> GSHMRIDPFKLAHWMNARKYTAAQTADLAGLPLDDLRRLLGDEANEPDPAAATALAEALSVEPSQLAADAHRNLTVVHKSAEEMHASRRPIQRDGIHFYNFYTLAAPEGRVAPVVLDILCPSDRLPALNNGHLEPAITVNLGPGDINGRWGEEITPQTWRVLHANHGGDRWITGDSYVEPSYCPHSYSLAGDAPARIVSYTAQSNISPLMTEANNWSTGAFEEALKALSGKVSAGSVLDLFLARRAHTRTSAAEAAGVPPADLEAALRSPASETGLTVLRTLGRALGFDYRVLLPADDQHDGVGKTWTTIEDSRRSRRTFGTYEAASMASAAHLPDLVGSFLRVDADGRGADLIDHAENHYVVTEGRLTLEWDG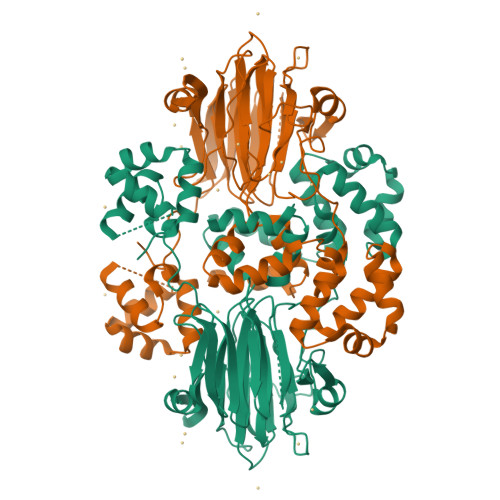PDGPASVELEPDGSAWTGPFVRHRWHGTGTVLKFGSGAHLGYQDWLELTNTFEPAATLRRGRRDLAGWGYDN>MRSRRVDVMDVMNRLILAMDLMNRDDALRVTGEVREYIDTVKIGYPLVLSEGMDIIAEFRKRFGCRIIADFKVADIPETNEKICRATFKAGADAIIVHGFPGADSVRACLNVAEEMGREVFLLTEMSHPGAEMFIQGAADEIARMGVDLGVKNYV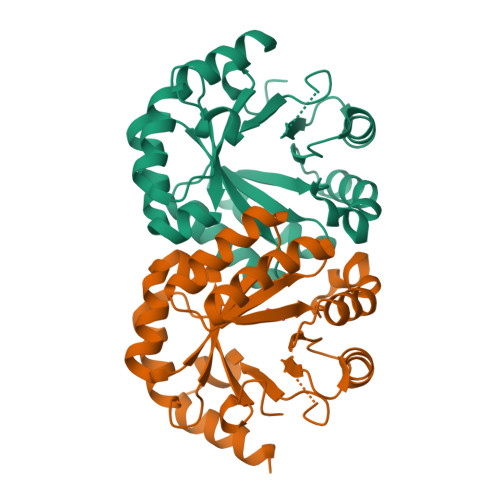GPSTRPERLSRLREIIGQDSFLISPGVGAQGGDPGETLRFADAIIAGRSIYLADNPAAAAAGIIESIKDLLNP[2x]>MGADDVVDSSKSFVMENFSSYHGTKPGYVDSIQKGIQKPKSGTQGNYDDDWEGFYSTDNKYDAAGYSVDNENPLSGKAGGVVKVTYPGLTKVLALKVDNAETIKKELGLSLTEPLMEQVGTEEFIKRFGDGASRVVLSLPFAEGSSSVKYINNWEQAKALSVELEINFETRGKRGQDAMYEYMAQACAGNRVRRSV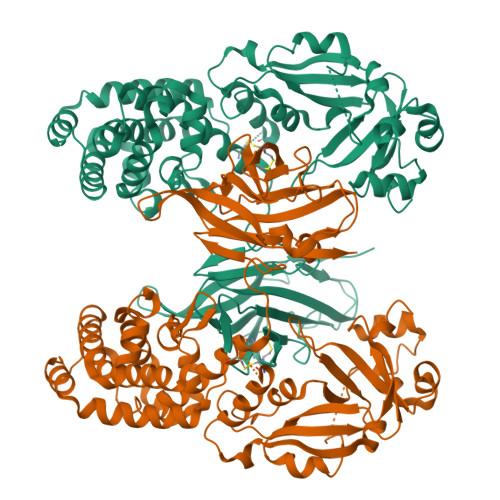GSSLSCINLDWDVIRDKTKTKIESLKEQGPIKNKMSESPNKTVSEEKAKQYLEEFHQTALEQPELSELKTVTGTNPVFAGANYAAWAVNVAQVIDSETADNLEKTTAALSILPGIGSVMGIADGAVHHNTEEIVAQSIALSSLMVAQAIPLVGELVDIGFAAYNFVESIINLFQVVHNSYNRPAYSPGHKTQPFLHDGYAVSWNTVEDSIIRTGFQGESGHDIKITAENTPLPIAGVLLPTIPGKLDVNKSKTHISVNGRKIRMRCRAIDGDVTFCRPKSPVYVGNGVHANLHVAFHRSSSEKIHSNEISSDSIGVLGYQKTVDHTKVNSKLSLFFEIKSMA[2x]>[2x]MGSSHHHHHHSSGRENLYFQGMCLSIP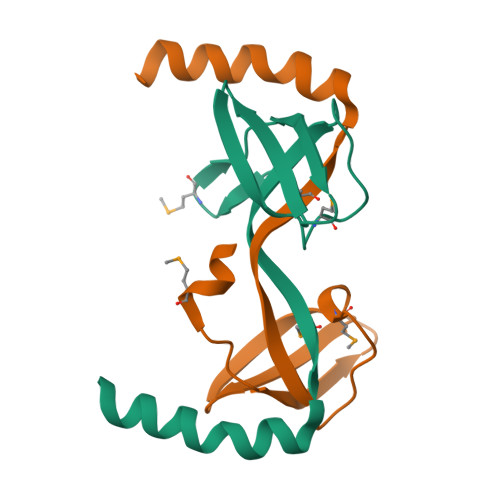SQVVAVDNERQSVTVDTLGVRRDVSSHLMTEPLAIGDYVLIHIGFVMNKIDRNDALQSLELYQEIVSKLENETTGS>[3x]MEQTEKSKVYAENGLLEKIKLCLSKKPLPSPTERKKFDHDFAISTSFHGIHNIVQNRSKIRRVLWLVVVLGSVSLVTWQIYIRLLNYFTWPTTTSIEVQYVEKMEFPAVTFCNLNRFQTDAVAKFGVIFFLWHIVSKVLHLQEITANSTGSREATDFAASHQNFSIVEFIRNKGFYLNNSTLLDCEFFGKPCSPKDFAHVFTEYGNCFTFNHGETLQAKRKVSVSGRGLSLLFNVNQEAFTDNPALGFVDAGIIFVIHSPKKVPQFDGLGLLSPVGMHARVTIRQVKTVHQEYPWGECNPNIKLQNFSSYSTSGCLKECKAQHIKKQCGCVPFLLPGYGIECDLQKYFSCVSPVLDHIEFKDLCTVGTHNSSCPVSCEEIEYPATISYSSFPSQKALKYLSKKLNQSRKYIRENLVKIEINYSDLNYKITQQQKAVSVSELLADLGGQLGLFCGASLITIIEIIEYLFTNFYWICIFFLLKISEMTQWTPPPQNHLGNKNRIEEC

The bile acid-sensitive ion channel (BASIC) is the least understood member of the mammalian epithelial Na+ channel/degenerin (ENaC/DEG) superfamily of ion channels, which are involved in a variety of physiological processes. There is, however, a conserved architecture among other members of the ENaC/DEG superfamily. These trimeric channels resemble a chalice in which a large extracellular domain (ECD) connects to a slender transmembrane domain (TMD) via linkers at the membrane interface. In this study, we used single-particle cryo-EM to determine the structure of hBASIC in the membrane-like environment of lipid nanodiscs, confirming its global adherence to the canonical ASIC fold. By determining structures in the presence and absence of Ca2+, we identified a single Ca2+-bound, non-conducting conformation of hBASIC, as well as both conducting and non-conducting conformations of Ca2+-free BASIC, revealing unexpected Ca2+-dependent conformational changes.

To reveal how hBASIC responds to Ca2+ removal, we prepared grids of hBASIC reconstituted in nanodiscs in the presence of 2 mM EGTA to chelate ambient Ca2+o and analyzed the sample using single-particle cryo-EM. Following extensive 3D classification methods, two predominant classes emerged, each containing between 15,000-20,000 particles. The overall resolution of both classes was lower than hBASIC in the presence of Ca2+, with both class 1 and class 2 having a global resolution of ~3.4 Å. In accordance with the electrophysiology data, we observed two distinct particle classes that differ in their pore conformations, which we thus refer to as ‘EGTA-closed’ (class 1), representing a non-conducting state, and ‘EGTA-open’ (class 2), representing an expanded, conducting state. In both the Ca2+-closed and EGTA-closed structures, this ‘glycine gate’ is impermeable to ions, with pore radii less than 1 Å and ~1.2 Å, respectively. Removal of Ca2+ promotes conformational heterogeneity in this molecular clutch. EGTA-closed resembles the Ca2+-closed conformation whereas EGTA-open is dramatically reorientated such that the positions of the L425 and N426 side chains are switched; N426 now facing the vestibule and L425 making contacts with the β1-β2 linker.> MSTSTYALRAGKRDVRREQQEIITRQINTAPYVQDAMMRVVVFAQYPSGRYKAFDYVFPDYLKVFLNWRELLEDTTTDYDPRTNTHRLMGQGYRQLIHPNHGSGEEPYDTRYPMGVIVSFNGNIDWTRARVEATNMHGLNNTDWREARAWGPHVICGNQLRKAGHLSRAVYVPLDEHNTVKVLATARQDGALNRFNGPQLAQTLTNNIVCPNVIEFNTESDVIDYAKMAHIAYIDQAGLIVASSDAYISGDSQA

Cypoviruses, members of the family Reoviridae, subfamily Spinareovirus, possess a single capsid layer with turrets and are commonly embedded in crystalline occlusion bodies called polyhedra, which are formed in the cell cytoplasm and mainly composed of a single virus-encoded protein, polyhedrin. To ensure the delivery of virus particles to the target intestinal cells, allowing the transmission of packages of infectious virus between hosts by oral-faecal routes, polyhedra are disrupted only when they are exposed to the very alkaline pH environment found in insect midguts. The fold of all the polyhedrins is highly similar – a β-barrel core sitting on a base domain, surrounded by a common array of five helices (H1–H5). The strongest intermolecular interactions define a trimer composed of a cluster of three β-barrels sandwiched by helices top and bottom.

All polyhedra belong to the same I23 space group and the native crystals (at 100 K) mostly possess a unit cell of 102–103 Å (102.8 ± 0.4 Å). The exceptions were CPV4, which forms crystals with 2 distinct unit cell dimensions (101.7 and 104.8 Å – the structure of the larger unit cell is an outlier and is discussed below), and CPV17 which has larger cell dimensions (106.1 Å room temperature and 104.9 Å 100 K). Native crystals of CPV4 polyhedra grouped into two distinct unit cell dimensions, 101.7 (±0.27) Å and 104.8 (±0.18) Å, whilst all SeMet crystals had the larger size. Crystals with both unit cell dimensions were observed on each of several frozen meshes suggesting that this was not an artefact of sample preparation. In the larger-cell structure, residues 1–12, 75–108, 189–192 and 254 were not visible, however SDS–PAGE analysis of crystals showed only a single protein band, corresponding to the full length polyhedrin, suggesting that this is not due to cleavage. Residues 75–108 and 189–192 are clustered around the centre of the dodecameric assembly described above. In the absence of these trimer–trimer interactions the trimers of the dodecamer slide away from teach other, enlarging the unit cell. The volume of the central cavity increases from 7220 Å3 to 18,784 Å3, and the solvent plus disordered protein fraction of the crystal becomes 41% (compared to a solvent content of 19% in the smaller cell crystals). Since residues 75–108 form the base domain we wondered if polyhedra crystals could be formed without the base domain. The CPV4Δ structure was very similar to that of CPV4 with the larger unit cell.(phenylmethyl) ~{N}-[(2~{R})-3-methyl-1-[[(2~{S})-1-[[(3~{S})-1-methylsulfanyl-4-oxidanylidene-pentan-3-yl]amino]-1-oxidanylidene-propan-2-yl]amino]-1-oxidanylidene-butan-2-yl]carbamate 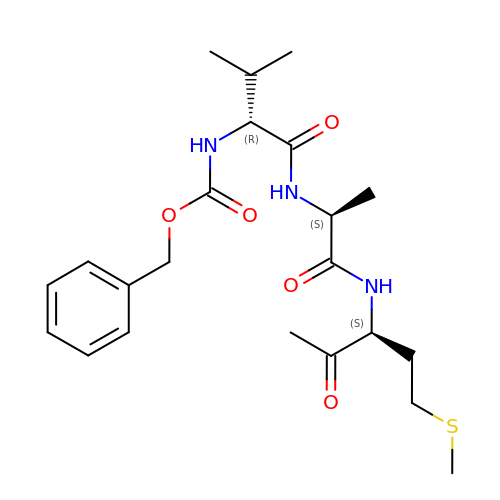| C22 H33 N3 O5 S | XQQSDBOJVLTWFC-ZYSHUDEJSA-N>PVWGCASTRGRSAEMEDASAAVPRFADVPVRLLASRRDL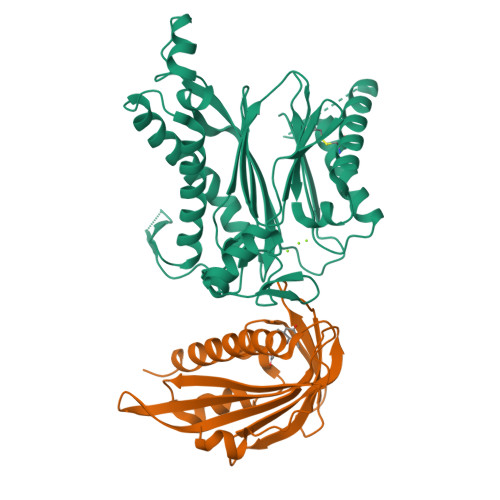DALGLDADALRLPAHLFGVFDGHGGAEVANYCRERIHVVLSAALARLGKNLGEMGEVDMKEHWDDVFTKCFQRVDDEVSGRVTRVVNGGGEVRSEPVTAENVGSTAVVALVCSSHVVVANCGDSRIVLCRGKEPVALSIDHKPDRKDERARIEAQGGKVIQWNGYRVFGMLAMSRSIGDRYLKPFVIPKPEVMVVPRAKDDDCLILASDGLWDVVSNEEACKVARRQILLWHKNNGAASPLSDEGEGSTDPAAQAAADYLMRLALKKGSEDNITVIVVDLKPRKKLKN[2x];>ETEYVRRFHRHEPRDHQCSSAVAKHIKAPVHLVWSLVRRFDQPQLFKPFVSRCEMKGNIEIGSVREVNVKSGLPATRSTERLELLDDNEHILSVRFVGGDHRLKNYSSILTVHPEVIDGRPGTLVIESFVVDVPEGNTKDETCYFVEALLKCNLKSLAEVSERLVVKDQTEPLDR[2x]> GSGSPLAQQIKNILSLIGQADAAGRMDEVRTLQLNLCQLMVEYFQQSDGDGGSPLAQQIQNIHSFGHQAWAAGRLDEVRRIQEN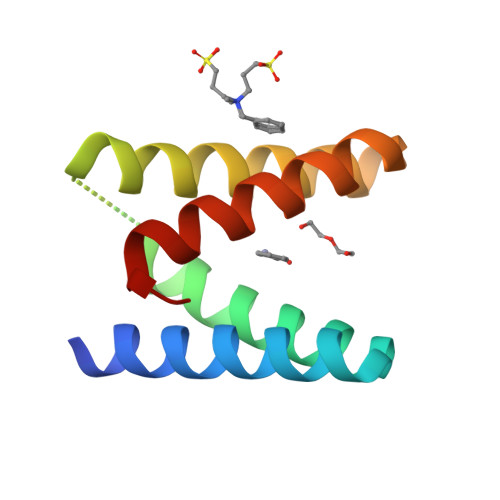LYQLMKEYFQQSD> ATITVSTPIKQIFPDDAFAETIKANLKKKSVTDAVTQNELNSIDQIIANNSDIKSVQGIQYLPNVRYLALGGNKLHDISALKELTNLGWLNLSNNQLETLPQGVFEKLTNLTTLNLSNNQL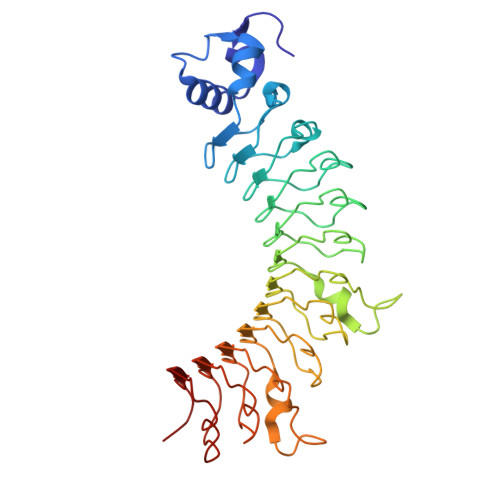TSLPQGVFERLASLTTLNLSNNNIANINDQMLEGLTNLTTLNLSHNNLARLWKHANPGGPIYFLKGLTNLTTLNLSSNGFDEIPREVFKDLTSLTTLNLSNNNIANINDQMLEGLTNLTTLNLSHNNLARLWKHANPGGPIYFLKGLTNLTTLNLSSNGFDEIPREVFKDLTSLTTLNLSNNQLTSLPQGVFERLTNLKTLNLSNNQLQS Organic Cation Transporter 1 (OCT1), a member of this family primarily localized on the basolateral membrane of hepatocytes, is involved in the uptake of cationic molecules for hepatic metabolism and excretion. Here, we present cryo-EM structures of full-length human OCT1 in the inward-open conformation, both ligand-free and drug-bound, indicating the basis for its broad substrate recognition. The overall architecture of OCT1 in our cryo-EM structures resembles the classical MFS transmembrane arrangement of pseudo-symmetric 6 + 6 transmembrane helical (TM) bundles corresponding to the N-terminal (TMs 1–6) and C-terminal (TMs 7–12) lobes. The structures also show a large extracellular domain (ECD) between TMs 1 and 2 unique to the SLC22 family.

The 6 + 6 TM bundles of our OCT1 cryo-EM structures are arranged in an inward-open conformation with the central substrate cavity accessible to the cytoplasm. Our cryo-EM map of OCT1-apo in the inward-open state defines the entire ECD, whereas this region was only partially resolved in the previous outward-open OCT3 and OCT1CS/OCT2CS structures, suggesting that the inward-open state restricts the flexibility of this domain. The core fold of the ECD is stabilized by three disulfide bonds: C50-C121, just after the anti-parallel beta sheet; C62-C102 towards the periphery of the ECD; and C88-C142 between the ECD and the start of TM2. We also observed additional density that likely corresponded to the first glycan sugars on residues N71, N96, and N112. In inward-open OCT1-apo, the complete closure of the extracellular gate was further stabilized by the union of hydrophobic residues from both lobes, shielding these residues from bulk solvent. Simulations of OCT1-apo revealed that residues V37, I365 and L366, which sit in the center of the hydrophobic gate, were within 3 Å of any solvent molecule for only 8.2%, 23.4% and 23.6% of the combined 1500 ns (n = 3 × 500 ns) of simulation time, respectively, suggesting these residues of the predicted hydrophobic gate were tightly packed, preventing extracellular solvent penetration between the N- and C- bundles. We did also observe weak cryo-EM density in the binding site of OCT1-apo at low thresholds (σ < 9). Although we were unable to determine the identity of this material, we hypothesize this may be a buffer component or an endogenous cationic ligand, or the average of multiple different chemical species, consistent with the well-established ability of OCT1 to bind a variety of ligands. Upon examination of E386 and D474, both residues were engaged in salt-bridge interactions with R439 and K214, respectively, as well as an ordered hydrogen-bonding network with surrounding residues.

> MPTVDDILEQVGESGWFQKQAFLILCLLSAAFAPICVGIVFLGFTPDHHCQSPGVAELSQRCGWSPAEELNYTVPGLGPAGEAFLGQCRRYEVDWNQSALSCVDPLASLATNRSHLPLGPCQDGWVYDTPGSSIVTEFNLVCADSWKLDLFQSCLNAGFLFGSLGVGYFADRFGRKLCLLGTVLVNAVSGVLMAFSPNYMSMLLFRLLQGLVSKGNWMAGYTLITEFVGSGSRRTVAIMYQMAFTVGLVALTGLAYALPHWRWLQLAVSLPTFLFLLYYWCVPESPRWLLSQKRNTEAIKIMDHIAQKNGKLPPADLKMLSLEEDVTEKLSPSFADLFRTPRLRKRTFILMYLWFTDSVLYQGLILHMGATSGNLYLDFLYSALVEIPGAFIALITIDRVGRIYPMAMSNLLAGAACLVMIFISPDLHWLNIIIMCVGRMGITIAIQMICLVNAELYPTFVRNLGVMVCSSLCDIGGIITPFIVFRLREVWQALPLILFAVLGLLAAGVTLLLPETKGVALPETMKDAENLGRKAKPKENTIYLKVQTSEPSGT> MFEARLVQGSILKKVLEALKDLINEACWDISSSGVNLQSMDSSHVSLVQLTLRSEGFDTYRCDR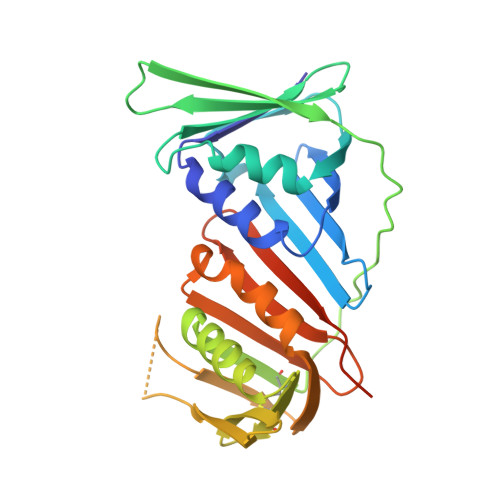NLAMGVNLTSMSKILKCAGNEDIITLRAEDNADTLALVFEAPNQEKVSDYEMKLMDLDVEQLGIPEQEYSCVVKMPSGEFARICRDLSHIGDAVVISCAKDGVKFSASGELGNGNIKLSQTSNVDKEEEAVTIEMNEPVQLTFALRYLNFFTKATPLSSTVTLSMSADVPLVVEYKIADMGHLKYYLAPKIEDEEGSLEHHHHHHH>[12x]XGEIAQ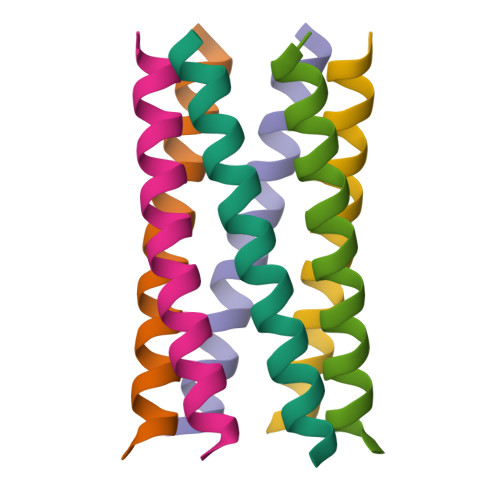TLKEIAKTLKEQAWTLKEIAQTLKGX> AFMPDARAYWVTSDLIAWNVGELEAQSVCLYASRAAAMSLSPSNGGIQGYDSKVELQPESAGLPETVTQKFPFISSYRAFRVPSSVDVASLVKCQLVVASFGADGKHVDVTGLQLPGVLDDMFAYTGPLGAVFSEDSVSLHLWAPTAQGVSVCFFDGPAGPALETVQLKESNGVWSVTGPREWENRYYLYEVDVYHPTKAQVLKCLAGDPYARSLSANGARTWLVDINNETLKPASWDELADEKPKLDSFSDITIYELHIRDFSAHDGTVDSDSRGGFRAFAYQASAGMEHLRKLSDAGLTHVHLLPSFHFAGVDDIKSNWKFVDECELATFPPGSDMQQAAVVAIQEEDPYNWGYNPVLWGVPKGSYASDPDGPSRIIEYRQMVQALNRIGLRVVMDVVYNHLDSSGPCGISSVLDKIVPGYYVRRDTNGQIENSAAMNNTASEHFMVDRLIVDDLLNWAVN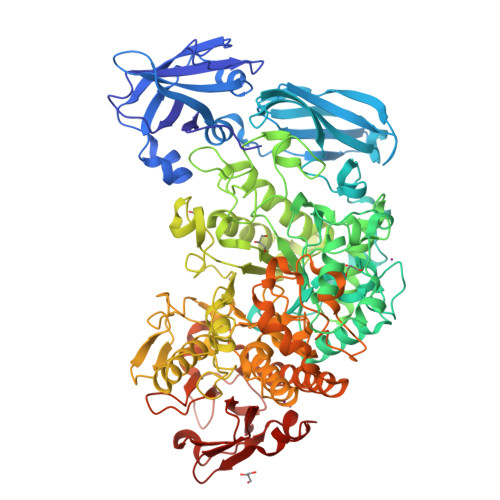YKVDGFRFDLMGHIMKRTMMRAKSALQSLTTDAHGVDGSKIYLYGEGWDFAEVARNQRGINGSQLNMSGTGIGSFNDRIRDAINGGNPFGNPLQQGFNTGLFLEPNGFYQGNEADTRRSLATYADQIQIGLAGNLRDYVLISHTGEAKKGSEIHTFDGLPVGYTASPIETINYVSAHDNETLFDVISVKTPMILSVDERCRINHLASSMMALSQGIPFFHAGDEILRSKSIDRDSYNSGDWFNKLDFTYETNNWGVGLPPSEKNEDNWPLMKPRLENPSFKPAKGHILAALDSFVDILKIRYSSPLFRLSTANDIKQRVRFHNTGPSLVPGVIVMGIEDARGESPEMAQLDTNFSYVVTVFNVCPHEVSMDIPALASMGFELHPVQVNSSDTLVRKSAYEAATGRFTVPGRTVSVFVEPRC> MAGSGVAKQIFALDFEIFGRVQGVFFRKHTSHEAKRLGVRGWCMNTRDGTVKGQLEAPMMNLMEMKHWL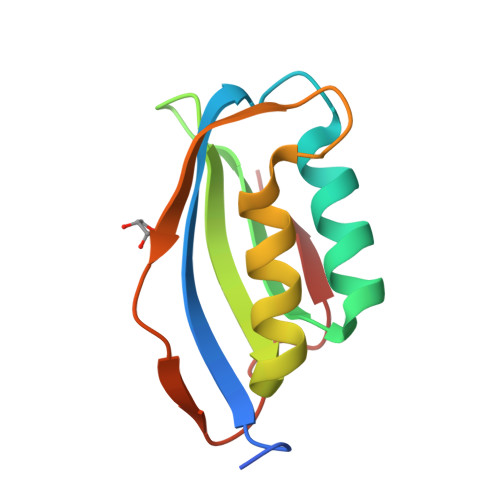ENNRIPNAKVSKAEFSQIQEIEDYTFTSFDIKH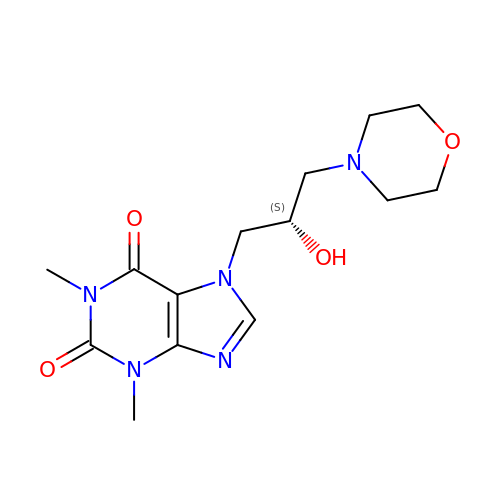7-[(2S)-2-hydroxy-3-(morpholin-4-yl)propyl]-1,3-dimethyl-3,7-dihydro-1H-purine-2,6-dione | C14 H21 N5 O4 | MPDQZYFYTXUHCN-JTQLQIEISA-N>TDLDAVRIKVDTVNAKPGDTVRIPVRFSGIPSKGIANCDFVYSYDPNVLEIIEIEPGELIVDPNPTKSFDTAVYPDRKMIVFLFAEDSG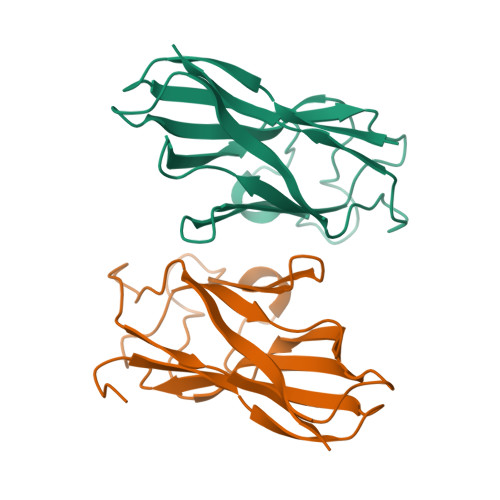TGAYAITEDGVFATIVAKVKSGAPNGLSVIKFVEVGGFANNDLVEQKTQFFDGGVNVG[2x]CD8 is expressed on the T-cell surface as dimers in two isoforms, the CD8αα homodimer and the CD8αβ heterodimer; both consist of an extracellular immunoglobulin variable (IgV) domain, a stalk region, a transmembrane domain and a cytoplasmic tail. Here, we report the high-resolution crystal structures of chicken, swine and bovine CD8α and confirm that they are capable of forming homodimers. All of them are CD8αα homodimers, and each CD8α exhibited a typical IgV architecture consisting of two anti-parallel sheets. Our results suggest that although CD8α and MHC I sequences change drastically during co-evolution, a few conserved key residues ensure that the CD8α forms dimers and interacts with p/MHC I during at least the co-evolution of endotherm species.

Three extracellular Ig-like domains of chicken, swine and bovine CD8α (cCD8α, sCD8α and bCD8α) were crystallized and diffracted to 2.0 Å, 1.8 Å and 1.8 Å, respectively. The sheets of CD8α are composed of 10 β strands, but there are 11 β strands in sCD8α and bCD8α because their A and G strands are divided into two separate parts. The two artiodactyl CD8αα dimers also have some distinct structural characteristics, and the most notable feature is that they have an additional A’ strand. The two artiodactyl sCD8αα can be discriminated from each other by certain characteristics, such as the longer A’ strand and shorter complementarity determining region 2 (CDR2) loop in sCD8αα. The buried surface areas (BSAs) of cCD8αα, sCD8αα, bCD8αα, mouse CD8αα (mCD8αα), rhesus macaque CD8αα (rCD8αα) and human CD8αα (hCD8αα) are 828.3 Å2, 979.6 Å2, 928.7 Å2, 1048.7 Å2, 1105.5 Å2 and 1026.3 Å2, respectively, indicating that they are tightly binding dimers. The BSAs of sCD8αα and bCD8αα are similar, but there are six hydrogen bonds in sCD8αα and only two hydrogen bonds in bCD8αα, indicating that CD8α dimerization does not mainly rely on hydrogen bonds. The Q residue on the C strand is involved in the formation of hydrogen bonds in five CD8αα dimers, but it was substituted by H in bCD8α, and no hydrogen bond is formed at this location in bCD8αα. The numbers of residues composing the cCD8αα, sCD8αα and bCD8αα cavities are 7, 7 and 9, and their volumes are 202.0 Å3, 322.9 Å3 and 384.6 Å3, respectively.

>[2x]SLSFRMSPTQKETRLGEKVELQCELLQSGMATGCSWLRHIPGDDPRPTFLMYLSAQRVKLAEGLDPRHISGAKVSGTKFQLTLSSFLQEDQGYYFCSVVSNSILYFSNFVPVFLP> AR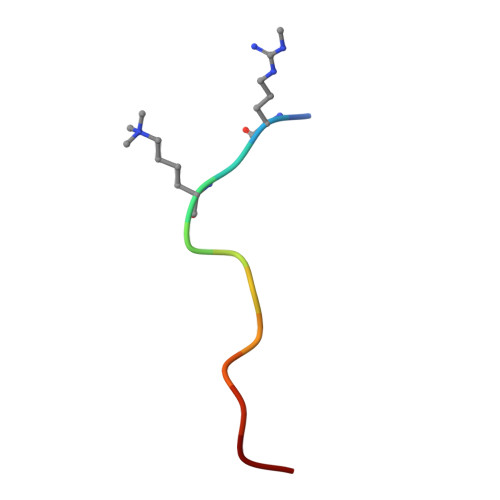TKQTARKAAG> SVALVPHVGMGLETRTETWMSSEGAWKHVQRIETW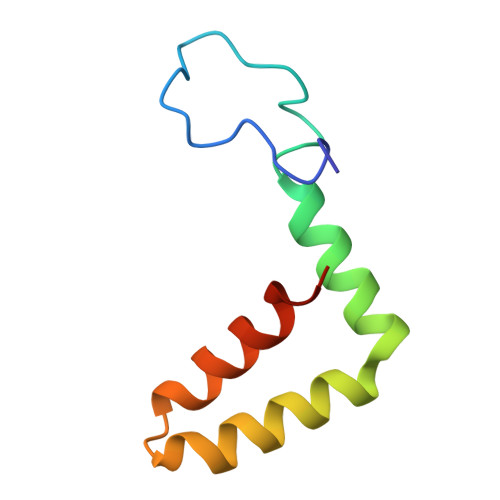ILRHPGFTMMAAILAYTIGTTHFQRALIFILLTAVTPSMT N-(2-AMINOETHYL)-N~2~-{(1S)-1-[4'-(AMINOSULFONYL)BIPHENYL-4-YL]-2,2,2-TRIFLUOROETHYL}-L-LEUCINAMIDE 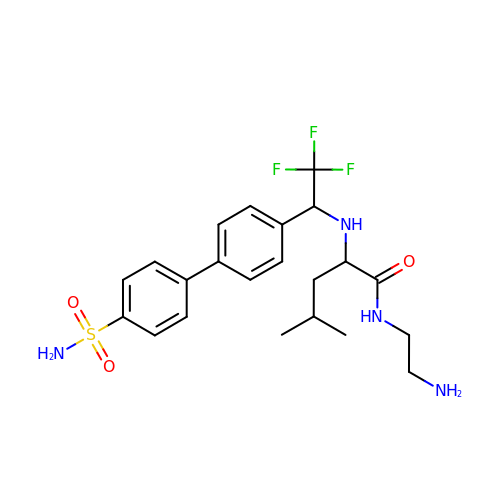| C22 H29 F3 N4 O3 S | QPXXBNKMAHUXBB-PMACEKPBSA-N>[2x]MMVLRMKVEWYLDFVDLNYEPGRDELIVEYYFEPNGVSPEEAAGRIASESSIGTWTTLWKLPEMAKRSMAKVFYLEKHGEGYIAKIA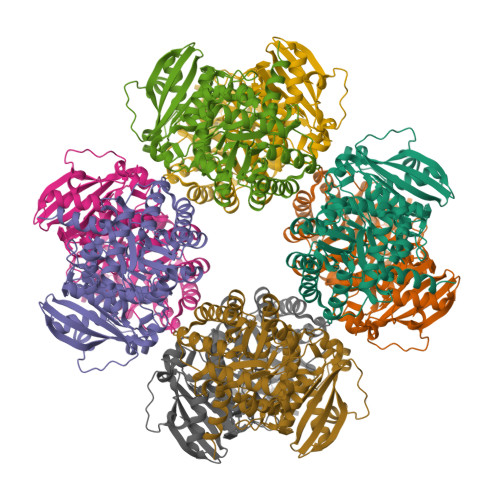YPLTLFEEGSLVQLFSAVAGNVFGMKALKNLRLLDFHPPYEYLRHFKGPQFGVQGIREFMGVKDRPLTATVPKPKMGWSVEEYAEIAYELWSGGIDLLKDDENFTSFPFNRFEERVRKLYRVRDRVEAETGETKEYLINITGPVNIMEKRAEMVANEGGQYVMIDIVVAGWSALQYMREVTEDLGLAIHAHRAMHAAFTRNPRHGITMLALAKAARMIGVDQIHTGTAVGKMAGNYEEIKRINDFLLSKWEHIRPVFPVASGGLHPGLMPELIRLFGKDLVIQAGGGVMGHPDGPRAGAKALRDAIDAAIEGVDLDEKAKSSPELKKSLREVGLSKAKVGVQH ALPHA-(2,6-DICHLOROPHENYL)-ALPHA-(2-ACETYL-5-METHYLANILINO)ACETAMIDE | C17 H16 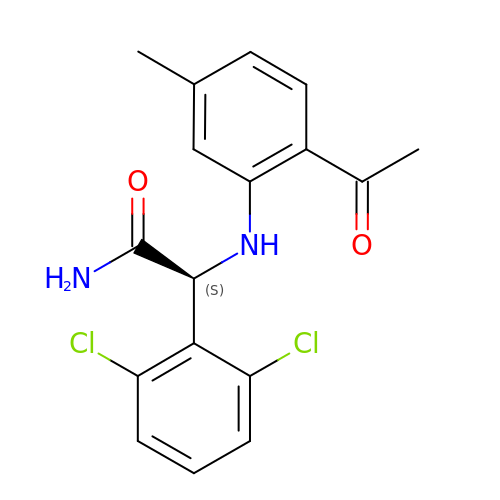Cl2 N2 O2 | CJPLEFFCVDQQFZ-INIZCTEOSA-N Among these, dUTPase and uracil DNA glycosylase enzymes are responsible for keeping DNA uracil-free. The enzyme dUTPase is tightly connected to this pathway, as dUMP is the sole precursor of de novo deoxythymidine triphosphate (dTTP) biosynthesis. For the protein dUTPase, there are numerous high-resolution dUTPase crystal structures deposited in the Protein Data Bank (PDB) (reviewed eg. in [2]). These structures all show the well-conserved dUTPase jelly-roll fold; however, there are some structural variations. Here we show that E. coli dUTPase and protein Stl form a strong protein complex associated with nanomolar dissociation constant.

However, we could successfully locate one specific position (EcDUTQ93) where mutation of the glutamine side-chain either into histidine or arginine led to strong inhibition of dUTPase activity by Stl. The two resulting mutant constructs (EcDUTQ93H and EcDUTQ93R) were both clearly inhibited by Stl and the inhibition resulted in a decrease of the steady-state velocity by 58% and 47%, respectively. Based on these data we observe that mutation of the 93rd glutamine position into either arginine or histidine increases the strength of interaction by approximately two-three fold. Therefore, we crystallized the EcDUTQ93H dUTPase mutant in the presence of the non-hydrolysable substrate analogue dUPNPP and compared its structure to the already deposited wild-type E. coli dUTPase structures. A novelty of our structure is that the whole C-terminal arm of the enzyme is visible in one of the subunits, whereas major parts of the segment are also visible in the other two subunits. This part of the enzyme has central role in catalysis, however it was so far missing from all existing E. coli dUTPase structures, even if they were crystallized in the presence of a substrate analogue. Our crystal structure provides a strong implication for existing interactions among the histidine point mutation at the 93rd position and the C-terminal arm of the enzyme, serving with a straightforward explanation for increased visibility of the C-terminal arm section. We hypothesized that the increased sensitivity of the EcDUTQ93H and EcDUTQ93R mutants for inhibition by protein Stl and their stronger Stl binding ability compared to the wild-type E. coli dUTPase is in connection with the restricted conformational freedom of the C-terminal arm of the enzyme. Data from the quenching experiments clearly argue that solvent accessibility of the tryptophan residue in the EcDUTQ93H,F145W dUTPase – dUPNPP complex is decreased as compared to the complex formed with EcDUTF145W. We therefore conclude that the quenching experiments in the solution state provide re-enforcement for the restricted conformational flexibility of the C-terminus observed in the crystal structure.

>[3x]MMKKIDVKILDPRVGKEFPLPTYATSGSAGLDLRACLNDAVELAPGDTTLVPTGLAIHIADPSLAAMMLPRSGLGHKHGIVLGNLVGLIDSDYHGQLMISVWNRGQDSFTIQPGERIAQMIFVPVVQAEFNLVEDFDATDRGEGGFGHSGRQ> GIDPFTVRTRVSEGLVLAEPAKLMISTDGSASTADL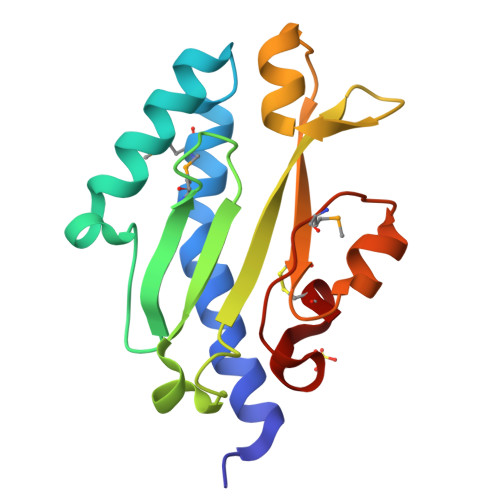TRATTTWNQQSNNLGASSKYVTSVLMDAGNTGVITITYVADQVGLPTAGNTLILSPYINDGNTRTALATAVAAGTRGTIDWACTSASNATATAQGFTGMAAGSVPQEFAPAQCR> GSHMGVQHKLDIFLVSEGIAIKEANLLKGDSYGCTIKIKLDKEKTFKFVIVLEPEWIDEIKPIYMKVNDESVELELDYKDAIKRIYSAEVVLSSDSVINLFSDVDVSYTSEYPTIKVNTIK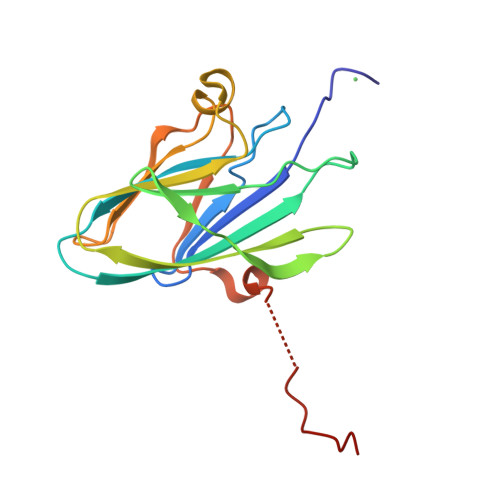KYYSVQNRGMTYVHIESPINTKDKSWFVEKNGWYEDRTHS>MSLRGELRVGLEPGYLPFEMKDKKGNVIGFDVDLAREMAKAMGVKLKLVPTSWDGLIPGLVTEKFDIIISGMTISQERNLRVNFVEPYIVVGQSLLVKKGLEKGVKSYKDLDKPELTLVTKFGVSAEYAAKRLFKNAKLKTYDTEAEAVQEVLNGK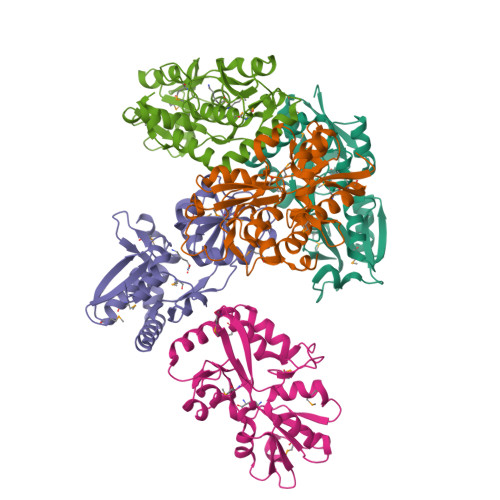ADMFIFDLPFNVAFMAQKGQGYLVHLDTSLTYEPLGWAIKKGDPDFLNWLNHFLAQIKHDGSYDELYERWFVDTKWLEKIQEGHHHHHH[6x]> GASPSAQELKEQGNRLFVGRKYPEAAACYGRAITRNPLVAVYYTNRALCYLKMQQHEQALADCRRALELDGQSVKAHFFLGQCQLEMESYDEAIANLQRAYSLAKEQRLNFGDDIPSALRIA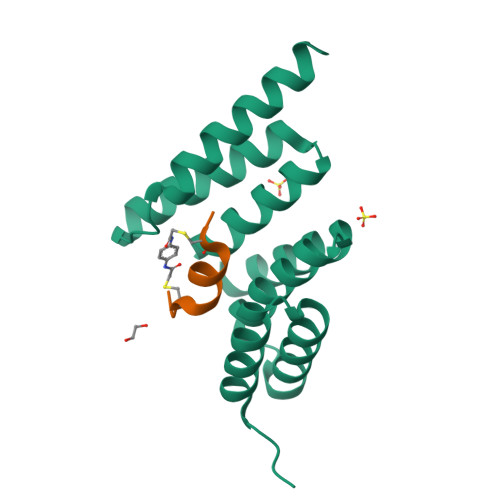KKKRWNSIEERR;> XPCYEAWVLCEYX>MAAATFHWDDPLLLDQQLADDERMVRDAAHAYAQGKLAPRVTEAFRHETTDAAIFREMGEIGLLGPTIPEQYGGPGLDYVSYGLIAREVERVDSGYRSMMSVQSSLVMVPIFEFGSDAQKEKYLPKLATGEWIGCFGLTEPNHGSDPGSMVTRARKVPGGYSLSGSKMWITNSPIADVFVVWAKLDEDGRDEIRGFILEKGCKGLSAPAIHGKVGLRASITGEIVLDEAFVPEENILPHVKGLRGPFTCLNSARYGIAWGALGAAESCWHIARQYVLDRKQFGRPLAANQLIQKKLADMQTEITLGLQGVLRLGRMKDEG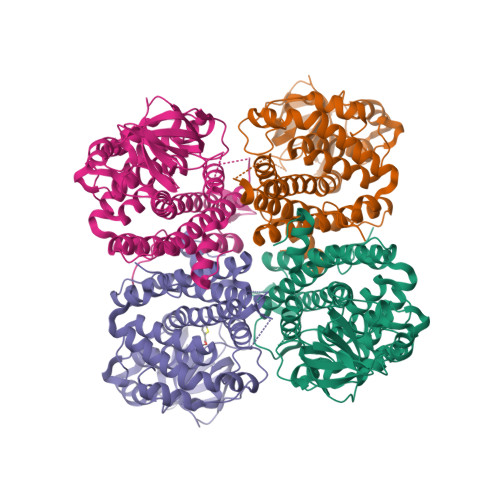TAAVEITSIMKRNSCGKALDIARLARDMLGGNGISDEFGVARHLVNLEVVNTYEGTHDIHALILGRAQTGIQAFF[4x]>[2x]EYGYIVTDQKPLSLA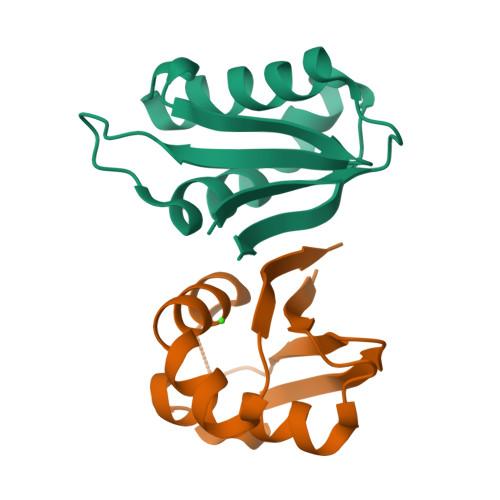AGVKLLEILAEHVHMSSGSFINISVVGPALTFRIRHNEQNLSLADVTQQAGLVKSELEAQTGLQILQTGVGQRE> TL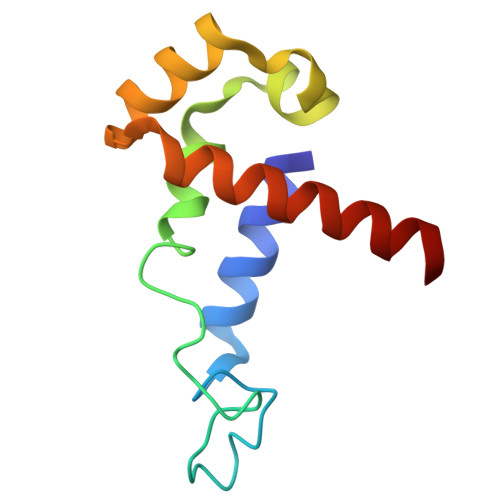DDFLEQLGQVRNMGPLDELLQMMPGAGKMKGLKNIQVDEKQLNHVEAIIKSMTVLEKEQPDIINASRRKRIAKGSGTSVQEVNRLLKQFDEMKKMMKQMT> LPTLGPGWQRQNPDPPVSRTRSLLLDAASGQLRLEDGFHPDAVAWANLTNAIRETGWAYLDLSTNGRYNDSLQAYAAGVVE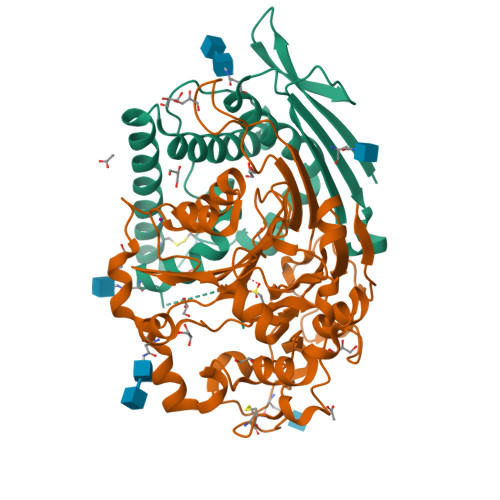ASVSEELIYMHWMNTVVNYCGPFEYEVGYCEKLKNFLEANLEWMQREMELNPDSPYWHQVRLTLLQLKGLEDSYEGRLTFPTGRFTIKPLGFLLLQISGDLEDLEPALNKTNTKPSLGSGS;> CSALIKLLPGGHDLLVAHNTWNSYQNMLRIIKKYRLQFREGPQEEYPLVAGNNLVFSSYPGTIFSGDDFYILGSGLVTLETTIGNKNPALWKYVQPQGCVLEWIRNVVANRLALDGATWADVFKRFNSGTYNNQWMIVDYKAFLPNGPSPGSRVLTILEQIPGMVVVADKTAELYKTTYWASYNIPYFETVFNASGLQALVAQYGDWFSYTKNPRAKIFQRDQSLVEDMDAMVRLMRYNDFLHDPLSLCEACNPKPNAENAISARSDLNPANGSYPFQALHQRAHGGIDVKVTSFTLAKYMSMLAASGPTWDQCPPFQWSKSPFHSMLHMGQPDLWMFSPIRVPWDGRGSHHHHHHG> RAITVFSPDGRLFQVEYAREAVKKGSTALGMKFANGVLLISDKKVRSRLIEQNSIEKIQLIDDYVAAVTSGLVADARVLVDFARISAQQEKVTYGSLVNIENLVKRVADQMQQYTQYGGVRPYGVSLIFAGIDQIGPRLFDCDPAGTIN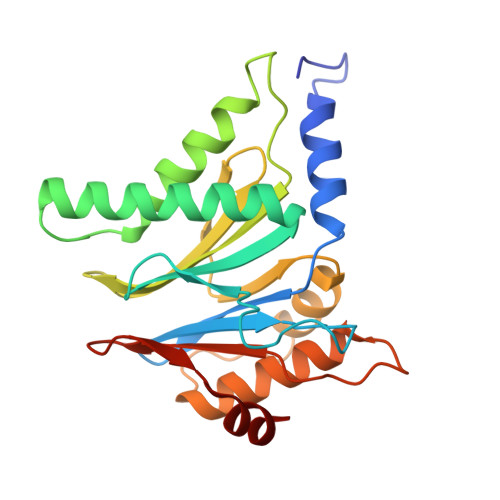EYKATAIGSGKDAVVSFLEREYKENLPEKEAVTLGIKALKSSLEEGEELKAPEIASITVGNKYRIYDQEEVKKFL>[2x]MRVYFDNNATTRVDDRVLEEMIVFYREKYGNPNSAHGMGIEANLHMEKARE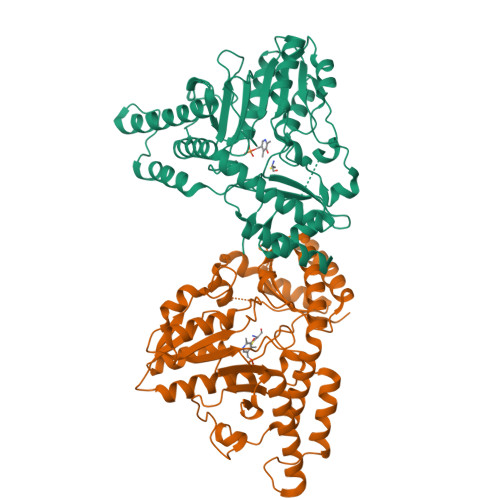KVAKVLGVSPSEIFFTSCATESINWILKTVAETFEKRKRTIITTPIEHKAVLETMKYLSMKGFKVKYVPVDSRGVVKLEELEKLVDEDTFLVSIMAANNEVGTIQPVEDVTRIVKKKNKETLVHVDAVQTIGKIPFSLEKLEVDYASFSAHKFHGPKGVGITYIRKGVPIRPLIHGGGQERGLRSGTQNVPGIVGAARAMEIAVEELSEAAKHMEKLRSKLVSGLMNLGAHIITPLEISLPNTLSVSFPNIRGSTLQNLLSGYGIYVSTSSACTSKDERLRHVLDAMGVDRRIAQGAIRISLCKYNTEEEVDYFLKKIEEILSFLDLTGNNRR> MNSHPRLTPWKSSDEV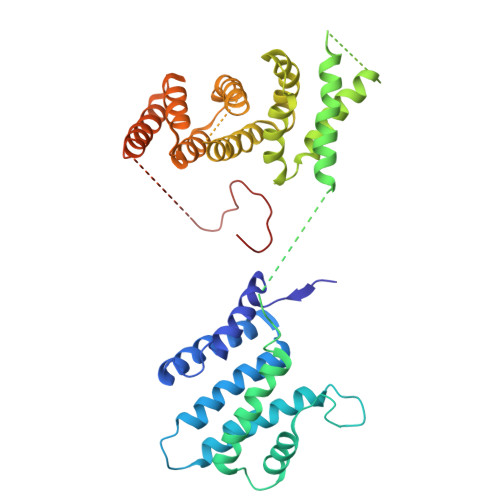VYLKGLFFPADREQISRDELYRQYEEAISLVEMYSSRTRVSHILQSTAHLFSALMMLESFEGGLDDTVRLTASMTIIRFVNGLLDPNQQSQFAIPLHLLAKKIDLPSLFVEFRHSATHDALPSLEMCKTCVDRAIDWVWDHYWDGVLSIVEPQVETDDLEESLIKELKDLFKQYRRIRRQNITKLYKFGDSTPEGKEYWTCIAGIKDHADMANFYNVMIERIVSNKLKWEHLRALFEPMMNHFIHLKGWDFPLGLIDSMLSKNYEYSKFRGIDDTERAYLNDQEFKCAQKWIRWLAIEQIDRYDDVLVSKMIDTLGKTNHELNVELLEKLQSRFSADPVIKDKIQAKLTLIQRLSTDTKTKRMNNLEDIMSDLESLKKRAKVTPTLHIKSFESHPNWTPKPFGVI> GPLGSVNSLEKHSWYHGPVSRSAAEYLLSSLINGSFLVRESESSPGQLSISLRYEGRVYHYRINTTADGKV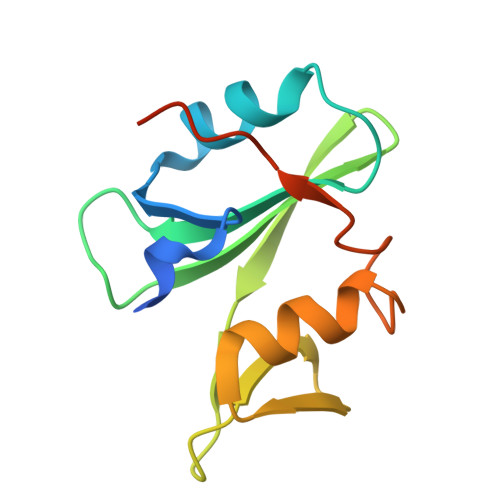YVTAESRFSTLAELVHHHSTVADGLVTTLHYPAPKCNKPTVYGIL>SMDRVFTTYKLMHTHQTVDFVRSKHAQFGGFSYKKMTVMEAVDLLDGLVDESDPDVDFPNSFHAFQTAEGIRKAHPDKDWFHLVGLLHDLGKVLALFGEPQWAVVGDTFPVGCRPQASVVFCDSTFQDNPDLQDPRYSTELGMYQPHCGLDRVLMSWGHDEYMYQVMKFNKFSLPPEAFYMIRFHSFYPWHTGRDYQQLCSQQDLAMLPWVREFNKFDLYT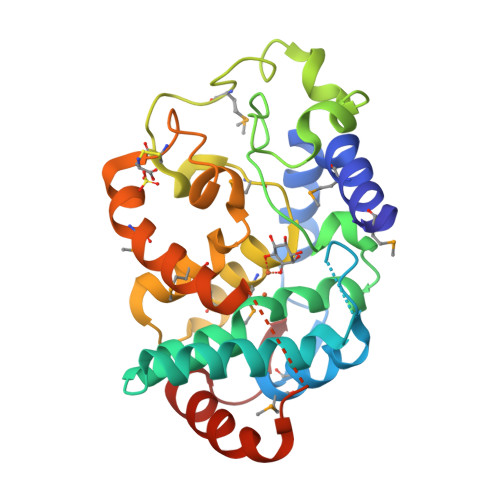KCPDLPDVDKLRPYYQGLIDKYCPGILSW[2x]>[2x]MNHKVHHHHHHIEGRHMRHIHLQVFGRVQGVGFRYF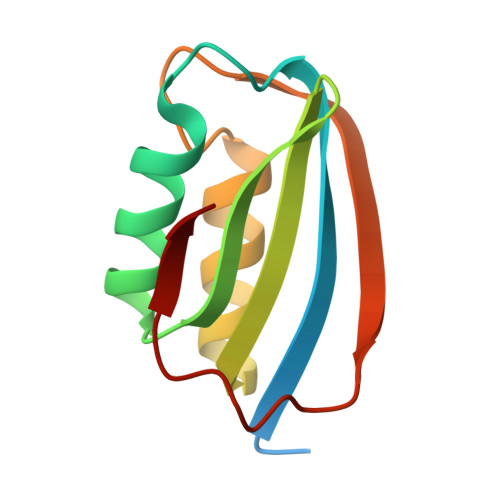TQRIAMNYNIVGTVQNVDDYVEIYAQGDDADIERFIQGVIEGASPASNVTSHQLEELELNQKLSDFRSI>AMSKKEININNYNDDAIQVLEGLDAVRKRPGMYIGSTDGAGLHHLVWEIVDNAVDEALSGFGDRIDVTINKDGSLTVQDHGRGMPTGMHAMGIPTVEVIFTILHAGGKFGQGGYKTSGGLHGVGSSVVNALSSWLEVEITRDGAVYKQRFENGGKPVTTLKKIGTAPKSKTGTKVTFMPDATIFSTTDFKYNTISERLNESAFLLKNVTLSLTDKRTDEAIEFHYENGVQDFVSYLNEDKEILTPVLYFEGEDNGFQVEVALQYNDGFSDNILSFVNNVRTKDGGTHETGLKSAITKVMNDYARKTGLLKEKDKNLEGSDYREGLAAVLSILVPEEHLQFEGQTKDKLGSPLARPVVDGIVADKLTFFLMENGELASNLIRKAIKARDAREAARKARDESRN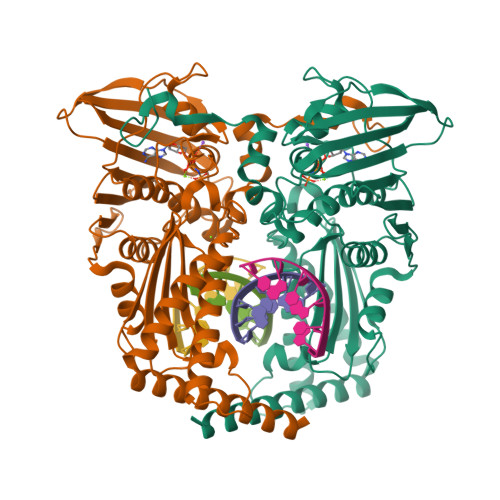GHHHHHH[2x]>[2x]SGISLDNSYKMDYPEMGLCIIINNKNFHKSTGMTSRSGTDVDAANLRETFRNLKYEVRNKNDLTREEIVELMRDVSKEDHSKRSSFVCVLLSHGEEGIIFGTNGPVDLKKITNFFRGDRCRSLTGKPKLFIIQACRGTELDC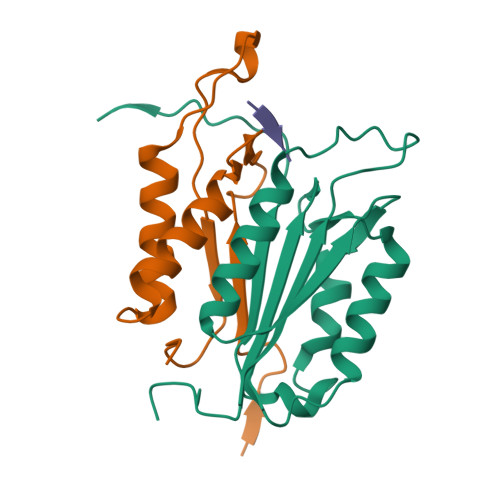GIETD;>[2x]SGVDDDMACHKIPVEADFLYAYSTAPGYYSWRNSKDGSWFIQSLCAMLKQYADKLEFMHILTRVNRKVATEFESFSFDATFHAKKQIPCIVSMLTKELYFYHHHHHHH;>[2x]XWEHD>[6x]MKCLFYIAGDVSNYSIVNYELNGQTQNTFFAAHALYNLFKPDKVIALIPDSLVKDNVSDEECYKNLVINRAKELNFAGMEEFMNKVEIRKIPNVGIASAI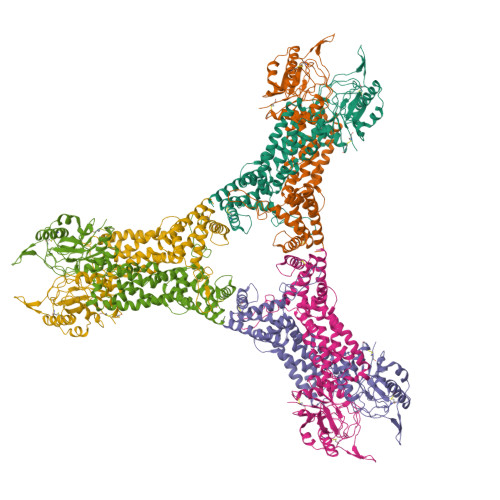QCENGAPKKEKNKEGREVLKRLPYNEKRSPIFIFNAIYAIFKDEACDEYLVDLTHGTNVLVSIGMNVGALFNAKFYSAPVMGMPGKDSIVNIVELTDVVQATNDSLMIRSSIENLDERYFKDYSAKLSRLNPTIFEEEEKKVLTRVKGTDVNVVINFLWNIRNGFTVNAVKSMNELKNIINQLEEDLEKLKSFYKNWEEHKNFQGETLLVLSDLDSTLKVKDLLIEGNDLEKLNYLLDLYIKASIYDKALSLARELPVAICLNKVGGGMFDDKNEKYKHCNEIVTSYLRLRYSGLMEFRNTLMHGGLSTDMKPNVDKDGNITPGKIVTKNKIEDFVKRELRNYFDKIVNFLSSA>[2x]MTSTTTTTETLQEAVPFVAPPSPPEDVNNKELPEKPYYDVEFNYRLDPRDGGDEVIWGGTVGLMRRKYETRTVRINNERGNEHNFNLDTHGFAWVKHKTSVTEFADYLAIRQGPYYGEVAEMLKRVTGATKVHVIGHLHRSLNYNDTTEEEKNAPDMTMTKGQTPGRFVHVDQSYQ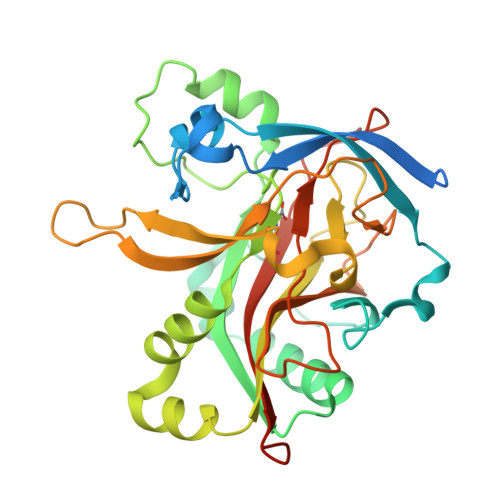GAVRRLYLDLPQEEARRLEKTRWAIINVWRPVRKVTNEPLAVCDARSVREDELFNTLHLVPMRWPDAAPQENQMWAVAPPKTPTQHKWHYVSGMTEDEALLIKMFDSKKDGTARRVPHSSFPTPDDFGEPRASTETRCFVFWEDQEAEALEHHHHHH> RYKKKWAATEPKFPAVRLALQNFDMTYSVQFGDLWPSIRVSLLSEQKYGALVNNFAAWDHVSAKLEQLSAKDFVNEAISHWELQSEGGQSAAPSPASWACSPNLRCFTFDRGDISRFPPARPGSLGVMEYYLMDAASLLPVLALGLQPGDIVLDLCAAPGGKTLALLQTGCCRNLAANDLSPSRIARLQKILHSYVPEEIRDGNQVRVTSWDGRKWGELEGDTYDRVLVDVPCTTDRHSLHEEENNIFKRSRKKERQILPVLQVQLLAAGLLATKPGGHVVYSTCSLSHLQNEYVVQGAIELLANQYSIQVQVEDLTHFRRVFMDTFCFFSSCQVGELVIPNLMANFGPMYFCKMRRLT;> XXXXXXXXXXXXXXXXXXXXXXXXXXXXXXQQLLDIISEFILLGLNPEPVCVVLKKSPQLLKLPIMQMRKRSSYLQKLGLGEGKLKRVLYCCPEIFTMRQQDINDTVRLLKEKCLFTVQQVTKILHSCPSVLREDLGQLEYKFQYAYFRMGIKHPDIVKSEYLQYSLTKIKQRHIYLERLGRYQ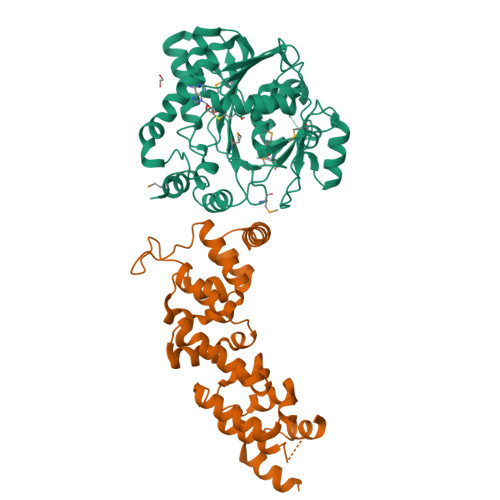TPDKKGQTQIPNPLLKDILRVSEAEFLARTACTSVEEFQVFKKLLAREEEESESS>MKGFAMLSIGKVGWIEKEKPAPGPFDAIVRPLAVAPCTSDIHTVFEGAIGERHNMILGHEAVGEVVEVGSEVKDFKPGDRVVVPAITPDWRTSEVQRGYHQHSGGMLAGWKFSNVKDGVFGEFFHVNDADMNLAHLPKEIPLEAAVMIPDMMTTGFHGAELADIQMGSSVVVIGIGAVGLMGIAGAKLRGAGRIIGVGSRPICVEAAKFYGATDILNYKNGHIVDQVMKLTNGKGVDRVIMAGGGSETLSQAVSMVKPGGIISNINYHGSGDALLIPRVEWGCGMAHKTIKGGLCPGGRLRMERLIDLVFYKRVD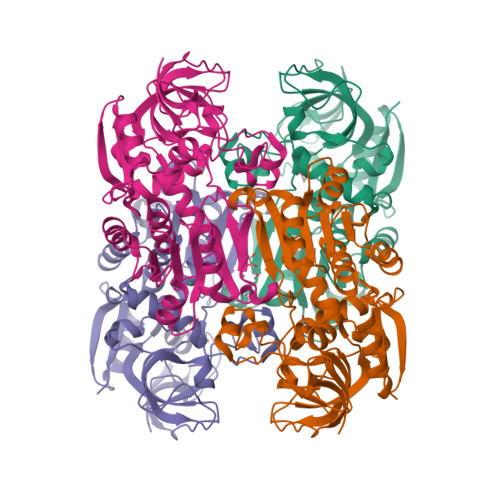PSKLVTHVFRGFDNIEKAFMLMKDKPKDLIKPVVILA[4x]>[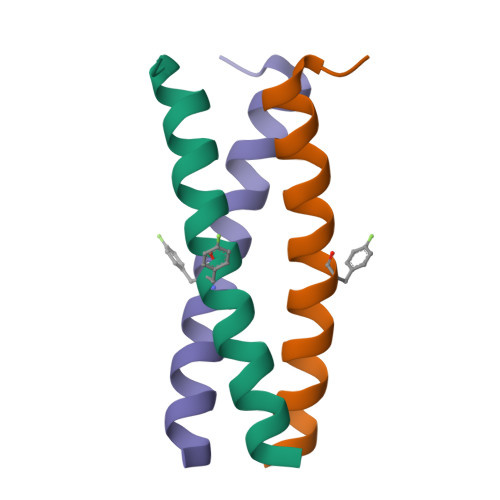2x]XEVEALEKKVEALEFKVQKLEKKVEALEHGWD> 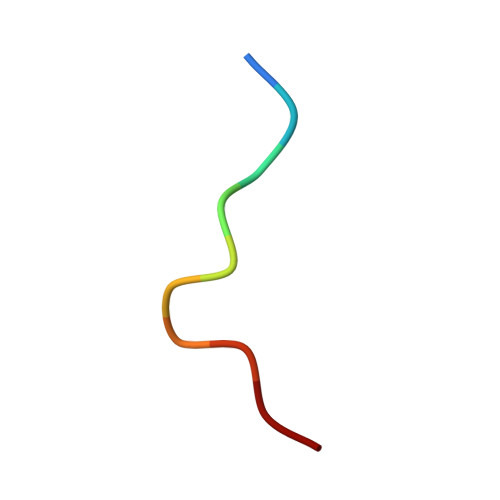KRKSRWDETP1-(3-METHYLPHENYL)-1H-BENZIMIDAZOL-5-AMINE | C14 H13 N3 | 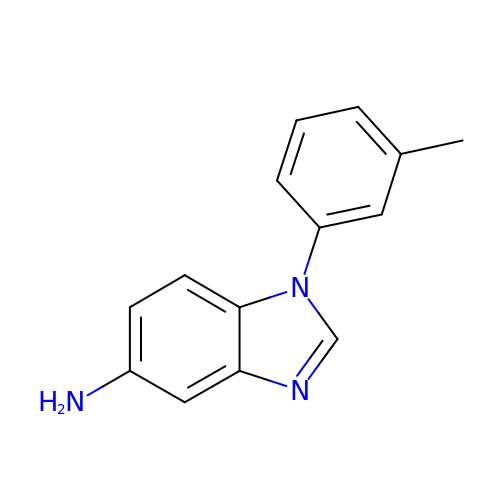VFSVFGIODYZMOF-UHFFFAOYSA-N>SNAMIIRPEQHWFLRLFDWHGAVLSKIIFRLLLNV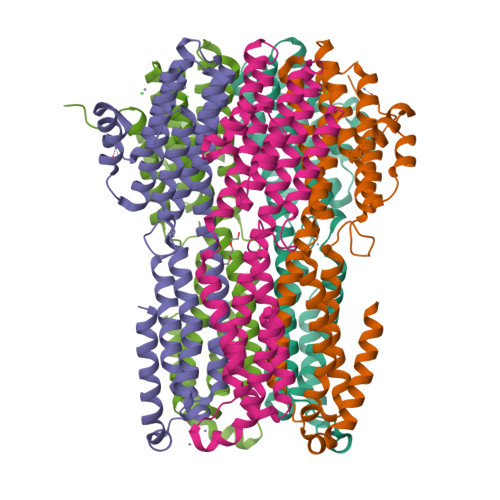LMSIIAIISYQWYEQLGIHLTVAPFSLLGIAIAIFLGFRNSASYSRFVEARNLWGTVLIAERTLVRQLRNILPAEHDAHRRIVSYLVAFSWSLKHQLRKTDPTADLRRLLPEERVTEILASSMPTNRILLLAGNEIGQLREAGKLSDITYGLMDNKLDELAHVLGGCERLATTPVPFAYTLILQRTVYLFCTLLPFALVGDLHYMTPFVSVFISYTFLSWDSLAEELEDPFGTAANDLPLNAMCNTIERNLLDMTGQHPLPE[5x]Recent work identifying the biosynthetic gene clusters for formycin A 1,11–13 pyrazomycin 2 (also known as pyrazofurin)14,15 and showdomycin 316 has laid the foundation for obtaining an enhanced understanding of two new enzymes (ForT and PyfQ), both of which catalyse C–C bond-forming steps in C-nucleotide biosynthesis. The function of ForT and PyfQ was originally assigned based on their homology to the enzyme (4-(β-d-ribofuranosyl)hydroxybenzene) (RHP) synthase, which mediates a key step in methanopterin biosynthesis. These enzymes all utilize 5′-phosphoribosyl-1′-pyrophosphate (PRPP) and an aromatic carboxylic acid to make the new C–C bond. The liberation of inorganic pyrophosphate and irreversible CO2 release provide the driving force for these reactions. The sequence of ForT is distantly related to homoserine kinase (<20% identity), a member of the GHMP kinase superfamily, although there are regions of strong sequence conservation.

The resulting crystals were soaked in 200 mM of PRPP 4 before data collection at the Diamond Light Source, allowing us to solve the structure of the ForT/PRPP complex to 2.5 Å resolution (ESI†).§ The crystal asymmetric unit contains a ForT monomer with residues 11–171, 180–205 and 209–341 (C-terminus) experimentally located in electron density; we assume that missing residues are located in conformationally disordered regions. The ForT monomer has three antiparallel β-sheets which form the core of the structure. Gel filtration and multi-angle light scattering suggests the enzyme to be a dimer in solution (ESI†), and the 2-fold rotation axis in the crystal does result in one (and only one) plausible dimer that relies on contacts between the helical bundles of each monomer. PRPP is located in the centre of the monomer, remote from the dimer interface. The 5′-phosphate of PRPP sits in a pocket and forms salt bridges with the side chains of Arg-19 and Arg-135; it also interacts with the N-terminus of short helix in the helical bundle. Hydrogen bonds are also observed between the 5′-phosphate and the side chains of Thr-106, Ser-139, Ser-142 and the backbone NH of Ser-142. The pyrophosphate moiety sits in different pocket and also makes a salt bridge with Arg-19. The pyrophosphate is hydrogen bonded to all seven backbone amides in a tight turn comprising residues His-99 to Ser-104 as well as with the side chain of His-99 and two water molecules. The ribose ring only makes one van der Waals contact with the side chain of Val-294. Informed by the crystal structure, we prepared a series of site-specific ForT variants by mutagenesis (ESI†) and used these variants in ITC measurements (ESI†), which confirmed that Arg-19, Thr-106 and Arg-135 are indeed essential for PRPP binding (ESI†).

> MALDRPDRSGAVRVSAPARLSFTLISLDGSSLRRNGIAAMAVDRPGLTAEVREAADGIVAVTGTAEETARELAAALEALRKLWDGPAARVDVLEALPQHSGFGSKTSTLLAVGHAYGRLCGVEPDLRELARTLGRGRTSGASTGLSAYGGFLVDGGHVNPPDFAEAPQKYLRPSRFAQQVAPPKPVVRLDFPDWPVLVLLTHGRHLGGQEELEWFHSVAPIPAEESWRTSHLVFMGLAPAVLEQDFDAFCAAVNEITFTGHFKQAQIAFQGDAVADVLEAGRAAPSVDAIALSVTGPACFAFTKRPEDAERWAWELKNRGLIRDFWFTRANNQGLATTVVS> MSENVEQHNPINAGTELSATGNESGGGGGG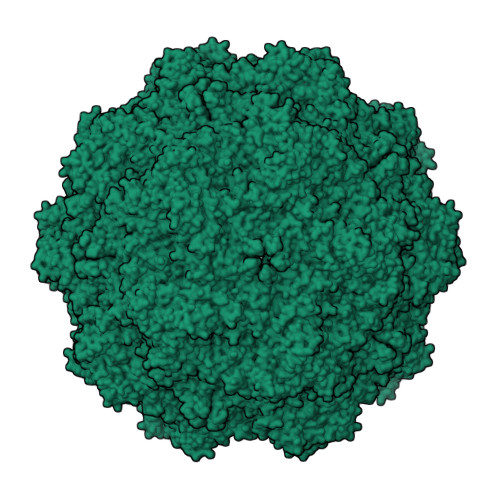GGGRGAGGVGVSTGTFNNQTEFQYLGEGLVRITAHASRLIHLNMPEHETYKRIHVLNSESGVAGQMVQDDAHTQMVTPWSLIDANAWGVWFNPADWQLISNNMTEINLVSFEQEIFNVVLKTITESATSPPTKIYNNDLTASLMVALDTNNTLPYTPAAPRSETLGFYPWLPTKPTQYRYYLSCIRNLNPPTYTGQSQQITDSIQTGLHSDIMFYTIENAVPIHLLRTGDEFSTGIYHFDTKPLKLTHSWQTNRSLGLPPKLLTEPTTEGDQHPGTLPAANTRKGYHQTINNSYTEATAIRPAQVGYNTPYMNFEYSNGGPFLTPIVPTADTQYNDDEPNGAIRFTMDYQHGHLTTSSQELERYTFNPQSKCGRAPKQQFNQQAPLNLENTNNGTLLPSDPIGGKSNMHFMNTLNTYGPLTALNNTAPVFPNGQIWDKELDTDLKPRLHVTAPFVCKNNPPGQLFVKIAPNLTDDFNADSPQQPRIITYSNFWWKGTLTFTAKMRSSNMWNPIQQHTTTAENIGNYIPTNIGGIRMFPEYSQLIPRKLY5-(morpholin-4-ylmethyl)quinolin-8-ol 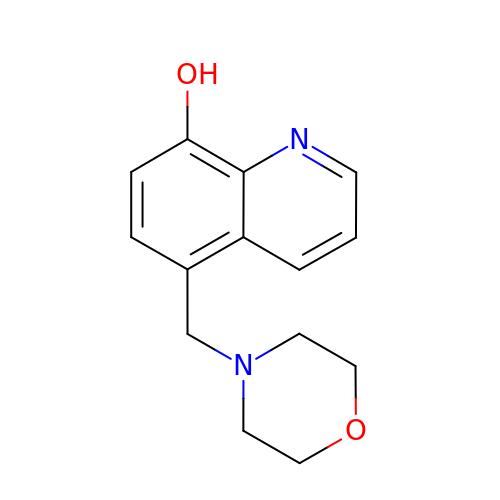| C14 H16 N2 O2 | AKUILKRKGZEPQD-UHFFFAOYSA-N>GSHMTIASVPTSRYLSDMTLEEMSRDWFMLMPRQKIIGPLCVRLDQAIMEKNIVLKANFSVIFNRLETLILLRAFTEEGAIVGEISPLPSLPGHTYEDVKNAVGVLIGGLEWNGNT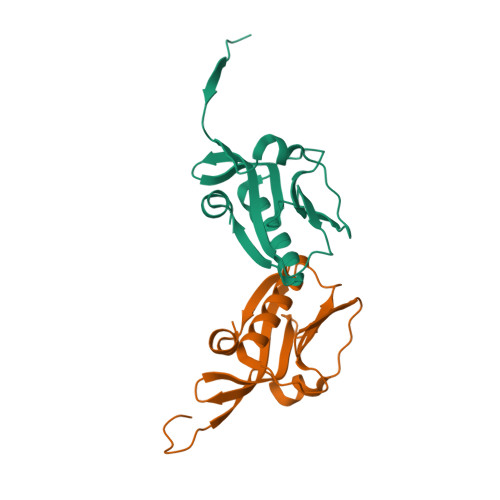VRVSENIQRFAWRNCDE[6x]>SANFTDKNGRQSKGVLLLRTLAMPSDTNANGDIFGGWIMSQMAMGGAILAKEIAHGRVVTVAVESMNFIKPISVGDVVCCYGQCLKVGRSSIKIKVEVWVKKVASEPIGERYCVTDAVFTFV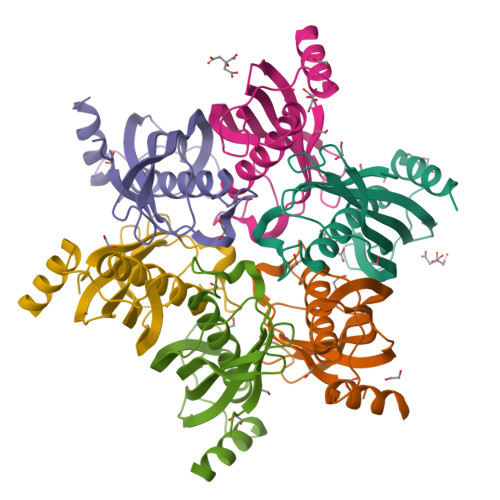AVDNNGRSRTIPRENNQELEKALALISEQPL[6x]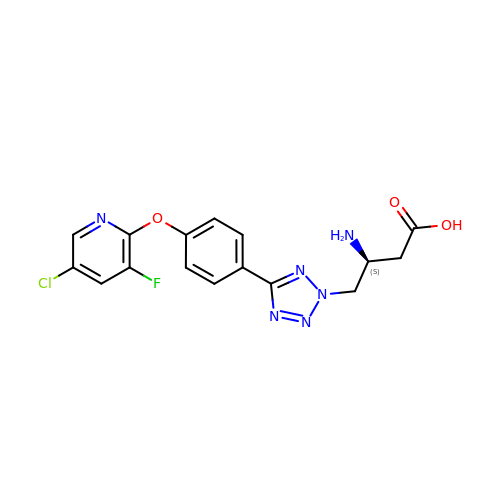(3~{S})-3-azanyl-4-[5-[4-(5-chloranyl-3-fluoranyl-pyridin-2-yl)oxyphenyl]-1,2,3,4-tetrazol-2-yl]butanoic acid | C16 H14 Cl F N6 O3 | ZEGMEJVULDALSH-NSHDSACASA-N> SNAATRLGEKLR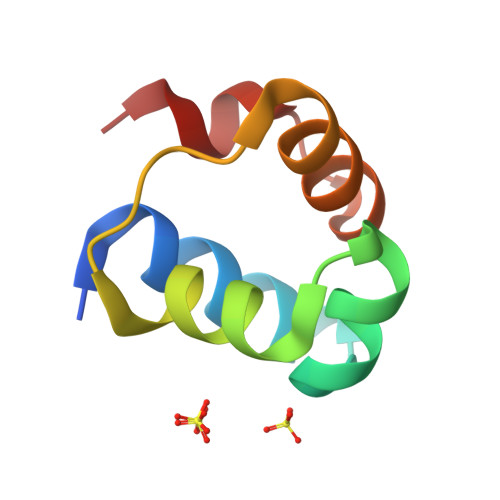DLRKQRGLTLEKLADMAGLSKSYLWELENRESQRPSAEKLTALADALGVGTSFFLED2,3,6-trifluoro-N-hydroxybenzamide | C7 H4 F3 N O2 | 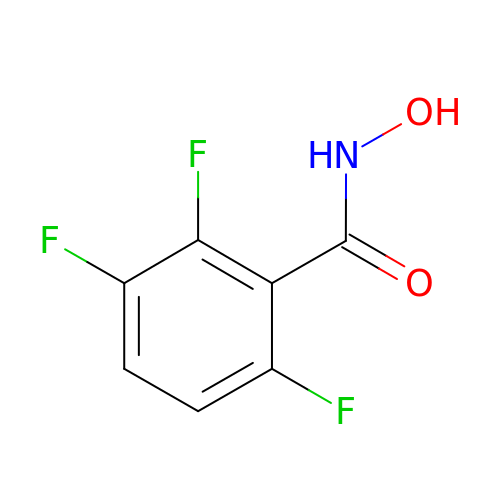YFACAFBGONHFNI-UHFFFAOYSA-N>QYVRIKNWGSGEILHDTLHHKATSDFTCKSKSCLGSIMNPKSLTRGPRDKPTPLEELLPHAIEFINQYYGSFKEAKIEEHLARLEAVTKEIETTGTYQLTLDELIFATKMAWRNAPRCIGRIQWSNLQVFDARNCSTAQEMFQHICRHILYATNNGNIRSAITVFPQRSDGKHDFRLWNSQLIRYAGYQMPDGTIRGDAATLEFTQLCIDLGWKPRYGRFDVLPLVLQADGQDPEVFEIPPDLVLEVTMEHPKYEWFQELGLKWYALPAVANMLLEVGGLEFPACPFNGWYMGTEIGVRDFCDTQRYNILEE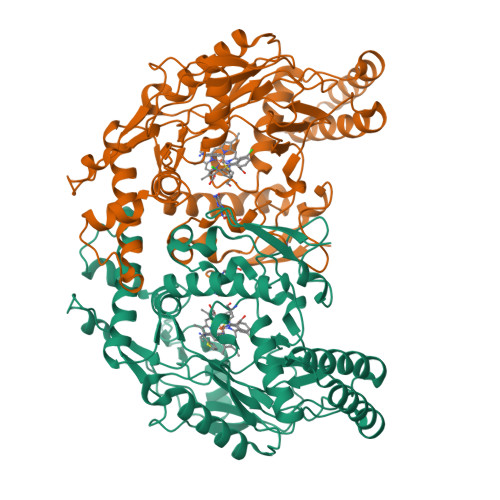VGRRMGLETHTLASLWKDRAVTEINVAVLHSFQKQNVTIMDHHTASESFMKHMQNEYRARGGCPADWIWLVPPVSGSITPVFHQEMLNYVLSPFYYYQIEPWKTHIW[2x]>SNAMSRGMSGLEDSSDLVVSPYVRMGGLTTDPVPTGGDDPHKVAMLGLTFDDVLLLPAASDVVPATADTSSQLTKKIRLKVPLVSSAMDTVTESRMAIAMARAGGMGVLHRNLPVAEQAGQVEMVKRSGGLLVGAAVGVGGDAWVRAMMLVDAGVDVLVVDTAHAHNRLVLDMVGKLKSEVGDRVEVVGGNVATRSAAAALVDAGADAVKVGVGPGSICTTRVVAGVGAPQITAILEAVAACRPAGVPVIADGGLQYSGDIAKALAAGASTAMLGSLLAGTAEAPGELIFVNGKQYKSYRGMGSLGAMRGRGGATSYSKDRYFADDALSEDKLVPEGIEGRVPFRGPLSSVIHQLTGGLRAAMGYTGSPTIEVLQQAQFVRITPAGLKESHPHDVAMTVEAPNYYAR[4x]

IMPDH catalyzes the NAD+-dependent conversion of inosine 5’-monophosphate (IMP) to xanthosine 5’-monophosphate (XMP), the first of the two step biosynthesis of guanosine 5’-monophosphate (GMP). Inosine 5’-monophosphate dehydrogenase (IMPDH) lies at a key intersection of the purine biosynthesis pathway and represents an extremely attractive target since it controls flux of the guanine nucleotide pool. We have overcome this major limitation by designing a variant that lacks the non-catalytic CBS subdomain (MtbIMPDH2ΔCBS), greatly improving solubility without impacting enzyme catalytic properties. Here we present the first crystal structures of MtbIMPDH2ΔCBS, including the apoenzyme, the E•XMP•NAD+ complex, and complexes with IMP and three inhibitors, MAD1, P41, and Q67.

The apo structure contains four polypeptide chains in the asymmetric unit (rmsds for Cα atoms of chain A versus other three are from 0.10 to 0.12 Å). A potassium ion is bound between subunits, interacting with six main chain carbonyls, three from the loop containing active site C341 (G336, G338, and C341) and three from the C-terminal portion of the adjacent subunit (E551’, S512’, and H513’). A phosphate ion originating from the crystallization buffer binds in the phosphate site of IMP, anchored by hydrogen bonding interactions with the backbone nitrogen atoms of S339, G376, G397 and S398 and the side chains of S339 and Y421. Thus the conformational dynamics of the active site flap may contribute to the differences in inhibitor affinities among IMPDHs from different sources. Interactions with the hypoxanthine moiety of IMP, E458, and AB-subsite are especially important for high affinity and selectivity. It is important to note that while the active site flap is partially disordered in all MtbIMPDH2ΔCBS structures, different conformations of the flap are observed in the apo structure and the structures of the complexes.> LEEK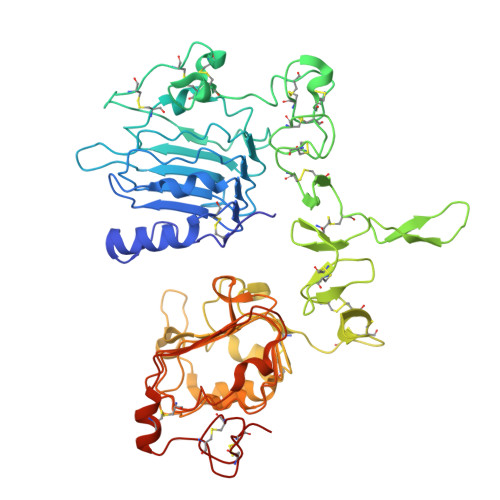KVCQGTSNKLTQLGTFEDHFLSLQRMFNNCEVVLGNLEITYVQRNYDLSFLKTIQEVAGYVLIALNTVERIPLENLQIIRGNMYYENSYALAVLSNYDANKTGLKELPMRNLQEILHGAVRFSNNPALCNVESIQWRDIVSSDFLSNMSMDFQNHLGSCQKCDPSCPNGSCWGAGEENCQKLTKIICAQQCSGRCRGKSPSDCCHNQCAAGCTGPRESDCLVCRKFRDEATCKDTCPPLMLYNPTTYQMDVNPEGKYSFGATCVKKCPRNYVVTDHGSCVRACGADSYEMEEDGVRKCKKCEGPCRKVCNGIGIGEFKDSLSINATNIKHFKNCTSISGDLHILPVAFRGDSFTHTPPLDPQELDILKTVKEITGFLLIQAWPENRTDLHAFENLEIIRGRTKQHGQFSLAVVSLNITSLGLRSLKEISDGDVIISGNKNLCYANTINWKKLFGTSGQKTKIISNRGENSCKATGQVCHALCSPEGCWGPEPRDCVSHHHHHH>SSQEYAYIDVDIN[4x];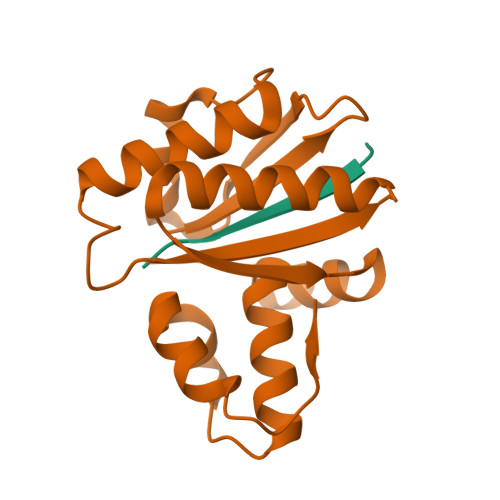>[4x]PSIGLVIDKKEKVIDAKPLNNDAKPILDEAAPKDMPLYDALSKILDISKKNGYINSADNIVLFSASINSGRNNVSESDKGIQEIISTLKDVAKDAGVKFEIIPSTEEDRQKALDQNLSMGRYAIYVKAVEEGVNLNLEDARNLSVSEILGKVNIGKFAISDT> MTSKTKNIDDIPPEIKEEMIQLYHDLPGIENEYKLIDKIGEGTFSSVYKAKDITGKITKKFASHFWNYGSNYVALKKIYV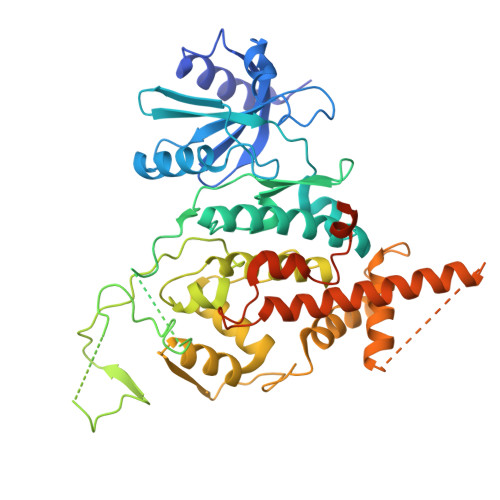TSSPQRIYNELNLLYIMTGSSRVAPLCDAKRVRDQVIAVLPYYPHEEFRTFYRDLPIKGIKKYIWELLRALKFVHSKGIIHRDIKPTNFLFNLELGRGVLVDFGLAEAQMDYKSMISSQNDYDNYANTNHDGGYSMRNHEQFCPCIMRNQYSPNSHNQTPPMVTIQNGKVVHLNNVNGVDLTKGYPKNETRRIKRANRAGTRGFRAPEVLMKCGAQSTKIDIWSVGVILLSLLGRRFPMFQSLDDADSLLELCTIFGWKELRKCAALHGLGFEASGLIWDKPNGYSNGLKEFVYDLLNKECTIGTFPEYSVAFETFGFLQQELHDRMSIEPQLPDPKTNMDAVDAYELKKYQEEIWSDHYWCFQVLEQCFEMDPQKRSSAEDLLKTPFFNELNENTYLLDGESTDEDDVVSSSEADLLDKDVLLISE Recently, a DNA pol from Thermococcus gorgonarius (Tgo), termed RT-H4 (hereafter referred to as Tgo-H4), has been developed with enhanced HNA RT activity. The aim of this study was to structurally characterize the mechanism of the laboratory-evolved reverse transcriptase Tgo-H4 (previously RT-H4) in interaction with its substrates, an HNA/DNA primer/template duplex and a bound triphosphate. As previous attempts to crystallize Tgo-H4 have been unsuccessful, we transferred its 18 mutations into the backbone of KOD DNA pol, which shares 93% sequence identity with the Tgo DNA pol (see Supplementary Figure S1 for sequence alignment) and had been successfully crystallized by us before. Just as Tgo-H4, Kod-H4 exhibits HNA reverse transcription activity, as was tested in 32P-based primer extension assays. All structures of KOD-H4 show the typical features of an archaeal DNA pol resembling a right hand with five distinct subdomains: N-terminal, 3′–5′-exonuclease (131–326), palm, finger (450–499) and thumb (588–774).

To gain insights into substrate binding and catalysis, we analyzed the two ternary complexes DNATP-KOD-H4 and HNA3+3TP-KOD-H4, both complexed with NHdGTP. Most striking is that in both ternary KOD-H4 structures (HNA3+3TP-KOD-H4 and DNATP-KOD-H4) the finger domain closes only partially upon TP binding. While the finger domain undergoes a closure of ∼25° from binary to ternary complex in the wt structure, it closes only by rotation around 7° and 11° in the HNA3+3TP-KOD-H4 and DNATP-KOD-H4 structures, respectively. As in the wt, the bound TP is located in the TP binding site in both ternary KOD-H4 structures. Although located in the same pocket, the TPs in both ternary KOD-H4 structures are shifted toward the O-helix. While in the wt the nucleobases of the base pair are co-planar within the incorporation site, a tilt is visible in both ternary KOD-H4 structures. For both HNA3+3TP-KOD-H4 and DNATP-KOD-H4, we observed open ternary complexes in which the distance from the primer end to the α-phosphate of the incoming TPs (4.8 and 5.0 Å, respectively) is significantly higher than the distance in the DNATP-KOD-wt (3.7 Å). This suggests that prior to catalysis, another conformational change may be required to bring the substrates closer together. Further, in KOD-wt, the backbone of A500 can interact with the phosphate backbone via a water molecule. In KOD-H4, A500 is mutated to a glutamate, which—at least in the structure of DNATP-KOD-H4—seems to establish a similar interaction via its side chain either directly or through a bound manganese ion.

> MILDTDYITEDGKPVIRIFKKENGEFKIEYDRTFEPYFYALLKDDSAIEEVKKITAERHGTVVTVKRVEKVQKKFLGRPVEVWKLYFTHPQDQPAIRDKIREHPAVIDIYEYDTPFAKRYLIDKGLVPMEGDEELKMLAFAIATLYHEGEEFAEGPILMISYADEEGARVITWKNVDLPYVDVVSTEREMIKRFLRVVKEKDPDVLITYNGDNFDFAYLKKRCEKLGINFALGRDGSEPKIQRMGDRFAVEVKGRIHFDLYPVIRRTINLPTYTLEAVYEAVFGQPKEKVYAEEITTAWETGENLERVARYSMEDAKVTYELGKEFLPMEAQLSRLIGQSLWDVSRSSTGNLVEWFLLRKAYERNELAPNKPDEKELARRRQKYEGGYVKEPERGLWENIVYLDFRSLYPSIIITHNVSPDTLNREGCGEYDVAPQVGHRFCKDLPGFIPSLLGDLLEERQKIKKKMKATIDPIERKLLDYRQRLIKILANSVYGHMGFENARWYCKECAESVTAWGREYLTMTIKEIEEKYGFKVIYSDTDGFFATIPGADAETVKKKAMEFLKYINAKLPGALELEYEGFYKRGFFVTKKKYAVIDEEGKITTRGLEIVRRDWSEIAKETQARVLEALLKDGDVEKAVRIVKEVTEKLSKYEVPPEKLVIHKQITRDLKDYKATGPHVAVAKRLAARGVKIRPGTVISYIVLKGSGRIGDRAIPFDEFDPTKHRYDAEYYIEKQVLPAVERILRAFGYRKEDLRYQKTRQVGLSAWLKPKGT> MLRFTRLFREMAPELQLEYMPVLFTRTILGPQGGFAGEERLVKLEVARKYMEAGHAVTPTEELRRGLWCYNPDTDKYDCFIERNEEFLDFAARKRQWLDVYWRVNTGYLLFGRQSWGQGFLINCPLRKRDVAQKLWEQYKVRIDPRLIEFREKDRRTGIQELGHNWCWLYLPGAEELGINREVYDNKRVKVRIHVRK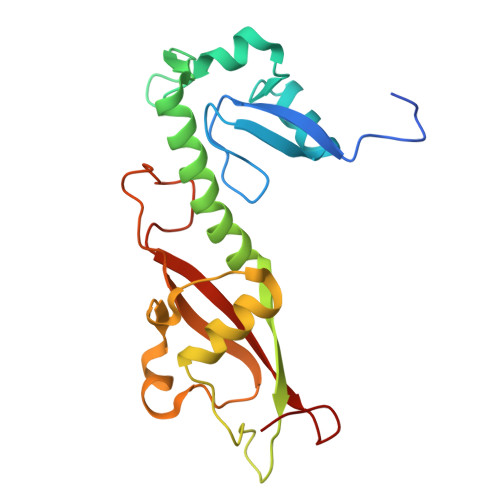MNSMFALY>MSRVLLCSAGHSSMVVPEAFHAVPEGFEEVHVFTTDSEKFNPVVLNDFFHSLPNVRFSITKCHGLADILNERDFEFYQEMLWQWYLTKMPDNELPYVCLSGGIKSMSASLQKAATLFGAQSVFHVLADNNPRNIEEMFDALQKGQIHFIEMGYEPGW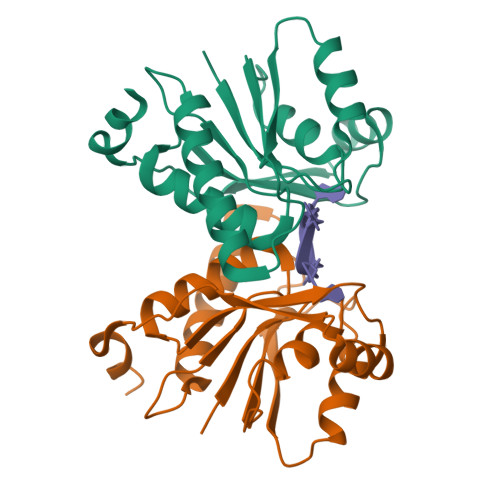AALRRLKKI[2x]>[2x]GNSATSADEQPHIGNYRLLKTIGKGNFAKVKLARHILTGKEVAVKIIDKTQLNSSSLQKLFREVRIMKVLNHPNIVKLFEVIETEKTLYLVMEYASGGEVFDYLVAHGRMKEKEARAKFRQIVSAVQYCHQKFIVHRDLKAENLLLDADMNIKIADFGFSNEFTFGNKLDT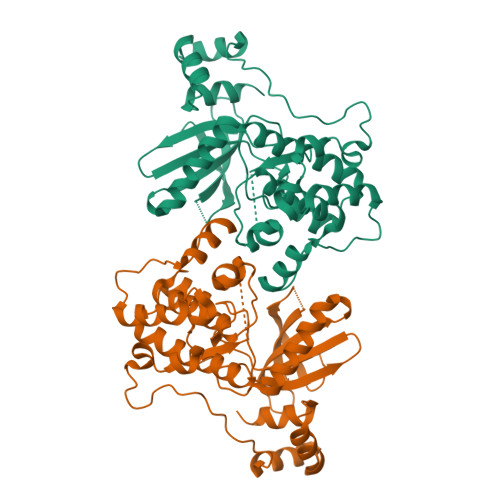FCGSPPYAAPELFQGKKYDGPEVDVWSLGVILYTLVSGSLPFDGQNLKELRERVLRGKYRIPFYMSTDCENLLKKFLILNPSKRGTLEQIMKDRWMNVGHEDDELKPYVEPLPDYKDPRRTELMVSMGYTREEIQDSLVGQRYNEVMATYLLLGYK3-[(1-ethanoylindol-3-yl)carbonylamino]-5-[[(2S)-oxan-2-yl]oxymethyl]benzoic acid | C24 H24 N2 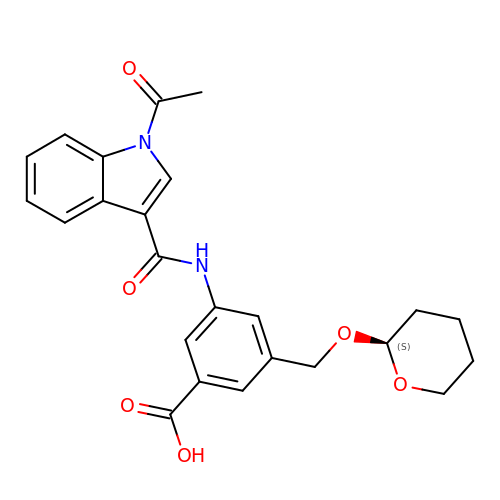O6 | MBYTWRXIPXJQJP-QFIPXVFZSA-N2-[1-(4,4-Difluorocyclohexyl)-piperidin-4-yl]-6-fluoro-3-oxo-2,3-dihydro-1H-isoindole-4-carboxamide | 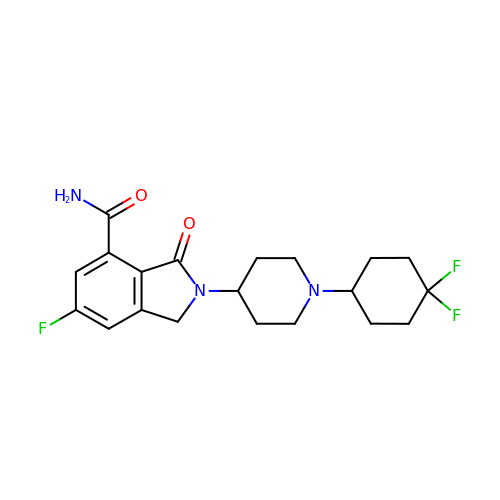C20 H24 F3 N3 O2 | ARYVAQSYRLZVQD-UHFFFAOYSA-N>METVSAVNQTLPISGGEPVKFTTYSAAVHKVLVMVNAGI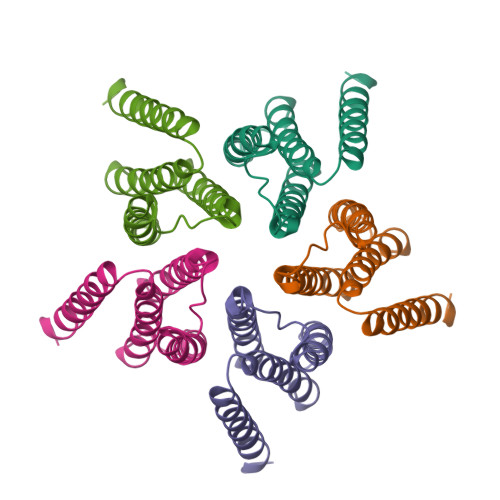LGLLQLVSQQSSVLETHKAAFLCFCVFILFYAVLRVREAMDVRLQPGLVPRLIGHGSHLFGGLAALVLVSVVSTAFSIVLFLLWFIWLSAVVYLETNKPSACPPQLPPV[5x]4-methyl-3-(4-piperidin-4-ylphenyl)-5-(3,4,5-trimethoxyphenyl)pyridine 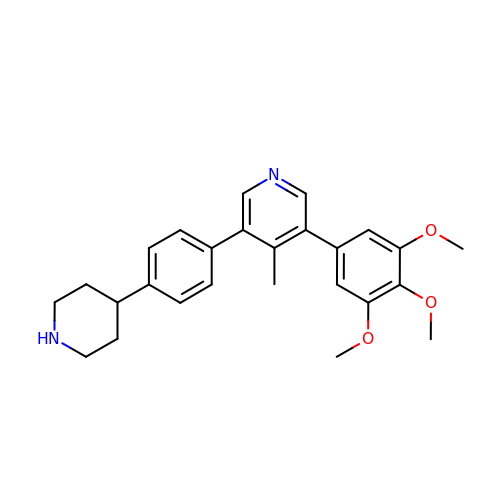| C26 H30 N2 O3 | WGZBSMWSGOJXPI-UHFFFAOYSA-N>[2x]SWTKEEEEALLDGMDLVKGPRW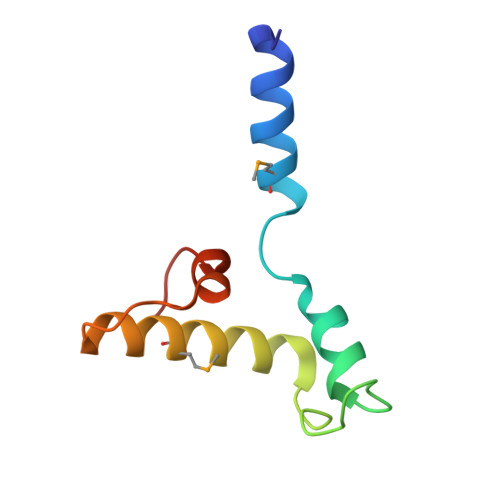SQILELYGPGGKKSEVLKYRNQVQLKDKARNMKLFFLKSGQVVPAALQCVTGDLRRD>[2x]MATVQPIVNSHLSELDEDVFHHFGFTTKSFDFKEKFGDVKFVCVCGSSGRIHNFAISMAKLAGLALPVENIAGSHARFVLYKVDHILFADHGIGIPSTLILMHEVTKLLYYAGCKDVLFIRLGTSDGLGVKPGTIVLSDRCVNTKLEPYNELCILGKPVRRQTKVDSNAVNE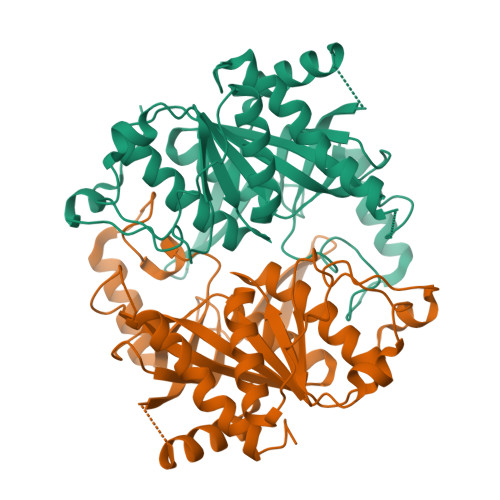LKKLSENLSLKCSVVVGGTITANDFYEELGRLNGSICTFSKEEKLAFLQSVYDHGIRNMEMEGAAITSHCYLTGHRAILVCVTVVNRLETDEVTTSTDEFKLFEQLPGQLVGEYLKRNNGIIVR> PMICLGLEGTAEKTGVGIVTSDGEVLFNKTIMYKPPKQGINPREAADHHAETFPKLIKEAFEVVDKNEIDLIAFSQGPGLGPSLRVTATVARTLSLTLKKPIIGVNHCIAHIEIGKLTTEAEDPLTLYVSGGNTQVIAYVSKKYRVFGETLDIAVGNCLDQFARYVNLPHPGGPYIEELARKGKKLVDLPYTVKGMDIAFSGLLTAAMRAYDAGERLEDICYSLQEYAFSMLTEITERALAHTNKGEVMLVGGV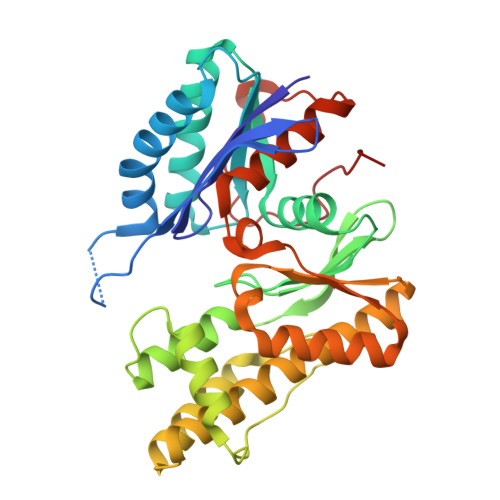AANNRLREMLKAMCEGQNVDFYVPPKEFCGDNGAMIAWLGLLMHKNGRWMSLDETKIIPNYRTDMVEVNWI>[2x]ALYEDPPDQKTSPSGKPATLKICSWNVDGLRAWIKKKGLDWVKEEAPDILCLQETKCSENKLP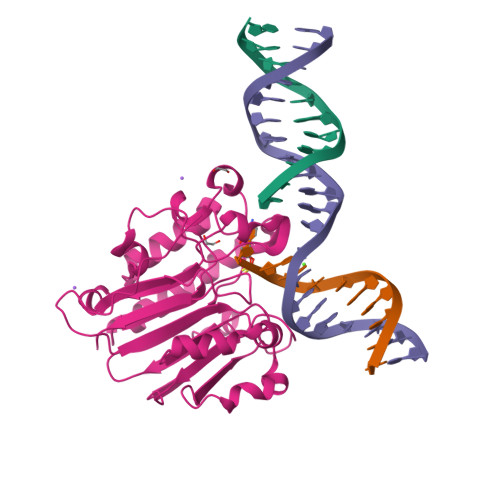AELQELPGLSHQYWSAPSDKEGYSGVGLLSRQAPLKVSYGIGDEEHDQEGRVIVAEFDSFVLVTAYVPNAGRGLVRLEYRQRWDEAFRKFLKGLASRKPLVLCGDLNVAHEEIDLRNPKGNKKNAGFTPQERQGFGELLQAVPLADSFRHLYPNTPYAYTAWTYMMNARSKNVGWRLDYFLLSHSLLPALCDSKIRSKALGSDHCPITLYLAL> GSHMLSDEQMQIINSLVEAHHKTYDDSYSDFVRFRPPVREGPVTRSASRAASLHSLSDASSDSFNHSPESVDTKLNFSNLLMMYQDSGSPDSSEEDQQSRLSMLPHLADLVSYSIQKVIGFAKMIPGFRDLTAEDQIALLKSSAIEIIMLRSNQSFSLEDMSWSCGGPDFKYCINDVTKAGHTLEHLEPLVKFQVGLKKLKLHEEEHVLLMAICLLSPDRPGVQDHVRIEALQDRLCDVLQAYIRIQHPGGRLLYAKMIQKLADLRSLNEEHSKQY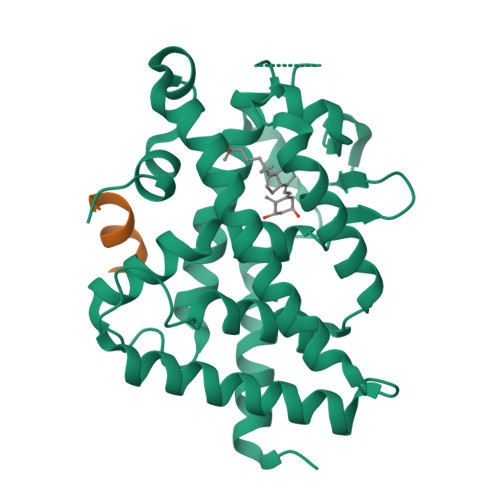RSLSFQPEHSMQLTPLVLEVFGSEVS;> RHKILHRLLQEGSPS> HHHHHHGSMAPKRSSDLFSQVVNSGPGSFLARQLGVPQPETLRRYRAGEPPLTGSLLIGGAGRVVEPLRAALEKDYDLVGNNLGGRWADSFGGLVFDATGITEPAGLKGLHEFFTPVLRNLGRCGRVVVVGGTPEAAASTNERIAQRALEGFTRSLGKELRRGATTALVYLSPDAKPAATGLESTMRFLLSAKSAYVDGQVFSVGADDSTPPADWEKPLDGKVAIVTGAARGIGATIAEVFARDGAHVVAIDVESAAENLAETASKVGGTALWLDVTADDAVDKISEHLRDHHGGKADILVNNAGITRDKLLANMDDARWDAVLAVNLLAPLRLTEGLVGNGSIGEGGRVIGLSSIAGIAGNRGQTNYATTKAGMIGITQALAPGLAAKGITINAVAPGFIETQ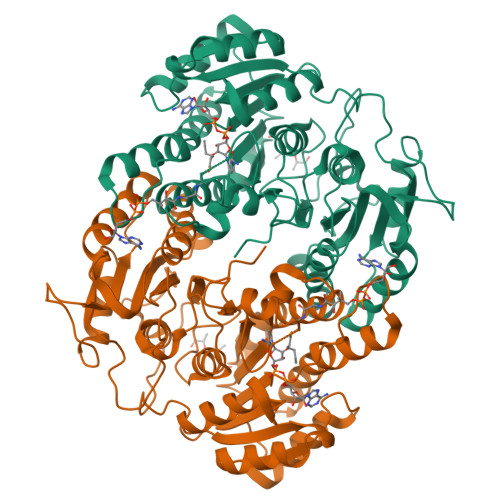MTAAIPLATREVGRRLNSLLQGGQPVDVAEAIAYFASPASNAVTGNVIRVCGQAMIGA The macromolecular SMN complex facilitates the formation of Sm-class ribonucleoproteins involved in mRNA processing (UsnRNPs). Here we report on the identification and structural determination of the SMN complex from the lower eukaryote Schizosaccharomyces pombe, consisting of SMN, Gemin2, 6, 7, 8 and Sm proteins. The core of the SMN complex is formed by several copies of SMN tethered through its C-terminal alpha-helices arranged with alternating polarity. This creates a central platform onto which Gemin8 binds and recruits Gemins 6 and 7.

To re-evaluate this interaction, an SpSMN fragment lacking its unstructured middle region (SpSMNΔ36–119) was co-expressed with a fragment of SpG2 lacking the N-terminus (SpG2ΔN80). We could detect clear electron density for SpSMNΔ36–119 but no electron density could be assigned to SpG2ΔN80, suggesting that the latter had dissociated and/or precipitated during crystallization. The structure revealed the SpSMN N-terminal G2 binding domain (residues 10–35) and the C-terminal YG-domain (residues 120–147) encompassing the YG-box and the serine-motif. Two molecules of SpSMNΔ36–119 in the asymmetric unit (termed the glycine–zipper dimeric unit), interact via the YG-box residues of interfacing helices. Interestingly, a closer inspection of the crystallographic packing showed that each glycine–zipper dimeric unit is stacked upon each other in an anti-parallel fashion around a screw axis between S130 and A134, leading to an infinite stacking along the crystallographic A axis. This interface, termed the anti-parallel interface, buries a surface area of 592 Å2 which is similar to the 620 Å2 buried surface area within the glycine–zipper interface. Anti-parallel stacking of glycine–zipper dimeric units is facilitated by the serine-motif where S130 and A134 pack against A134 and S130, respectively, of the interfacing helix of the adjacent dimeric unit, through mainchain atoms. The methyl group of each A134 forms hydrophobic contacts with the W131 sidechain of the interfacing helix. The sidechains of each W131 are stabilized by hydrogen bonding to the interfacing T138 sidechains. Our results thus corroborate the previous notion that the SMN glycine–zipper dimers are the fundamental unit of higher order oligomers and reveal a novel anti-parallel interface between glycine–zipper dimers required for higher order oligomer formation.

>MGDQSQKEVWDDSELRNAFETALHEFKKYHSIEAKGYDETYKKLIMSWYYAGYYTGLAEGLAKSEQRKD[2x]>[2x]PSVYDAAAQLTADVKKDLRDSWKVIGSDKKGNGVALMTTLFADNQETIGY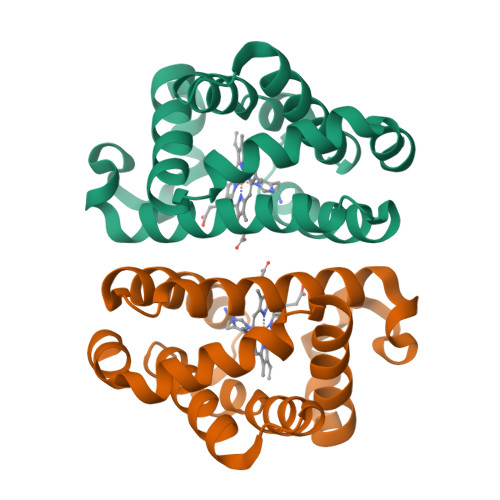FKRLGNVSQGMANDKLRGHSITLMYALQNFIDQLDNPDDLVCVVEKFAVNHITRKISAAEFGKMNGPIKKVLASKNFGDKYANAWAKLVAVVQAAL> AEESRKRLRFARLSEHATAPTKGSERAAGYDLYSAYDYTVLPMEKAIVKTDIQIALPSGCYGRVAPRSGLAAKHFIDVGAGVIDEDYRGNVGVVLFNFGKEKFEVKKGDRIAQLICERIFYPEIEEVQVLDDTERGSGGFGSTGTNLEHHHHHHH

Deoxyuridine 5'-triphosphate nucleotidohydrolase (dUTPase, EC 3.6.1.23) is a ubiquitous enzyme in DNA repair that plays a key role in preventing uracil from being incorporated into DNA. dUTPases are widespread in organisms, including eukaryotes, prokaryotes, and some viruses. On the one hand, it catalyzes the cleavage of dUTP into dUMP and pyrophosphate (PPi), which reduces the possibility that dUTP will be incorporated into DNA through DNA polymerase. Herein, we determine the crystal structures of ASFV dUTPase and swine dUTPase in both their ligand-free and ligand-bound forms. We observe that the swine enzyme employs a classical dUTPase architecture made up of three-subunit active sites, whereas the ASFV enzyme employs a novel two-subunit active site.

The prokaryotic expression of full-length swine dUTPase was difficult, so an N-terminal truncated form of sDUT (residues 54–221) was expressed. In contrast to ASFV dUTPase, swine dUTPase (sDUT) is a classical dUTPase. The α,β-bridging oxygen in dUTP was replaced by an imido group to form 2′-deoxyuridine 5′-(α,β-imido) triphosphate (dUPNPP), a nonhydrolyzable substrate analog and potent competitive inhibitor of dUTPase. The sDUT-dUPNPP-Mg2+ complex structure represents the prereaction state of the substrates just after binding to the active site. The swine dUTPase active site is inseparable from the trimer assembly as follows: one subunit provides catalytic motifs I, II, and IV; another subunit provides motif III; and another subunit provides motif V. In detail, as β12 is antiparallel to β3 and β7, the C-terminal β-strand (β13) is swapped to the adjacent subunits, and eventually, the C-terminal motif V reaches the active site opposite of its own subunit. For example, in swine dUTPase, the corresponding four amino acids are Cys, Glu, Arg, and Ile, and these motif IV–corresponding amino acids form a long β-strand (β12). The Arg193 at the end of β12 forms hydrogen bonds with an adjacent Arg193, and this rigid structure fixes the direction of subsequent amino acids, which ensures that the C-terminal β-strand (β13) is swapped into a neighboring subunit. Moreover, both Met99 of ASFV dUTPase and Gly167 of swine dUTPase offer main-chain oxygen and nitrogen atoms rather than side-chain atoms for hydrogen bonds with the uracil. There is 90% genetic similarity between swine dUTPase and human dUTPase, and their five conserved motifs were also consistent.> SINDSKILSLQNKKNALVDTSGYNAEVRLEGDVQVNTIYTNDFKLSSSGDKIIVNLNNNILYSAIYENSSVSFWIKISKDLTNSHNEYTIINSIKQNSGWKLCIRNGNIEWILQDINRKYKSLIFDYSESLSHTGYTNKWFFVTITNNIMGYMKLYINGELKQSERIEDLDEVKLDKTIVFGIDENIDENQMLWIRDFNIFSKELSNEDINIVYEGQILRNVIKDYWGNPLKFDTEYYMIN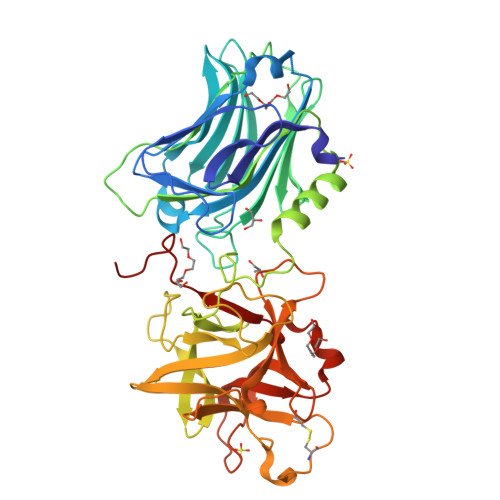YNYIDRYIAPKNNILVLVQYSDISKLYTKNPITIKSAANKNPYSRILNGDDIMFHMLYDSREYMIIRDTDTIYATQGGQCSKNCVYALKLQSNLGNYGIGIFSIKNIVSQNKYCSQIFSSFMKNTMLLADIYKPWRFSFENAYTPVAVTNYETKLLSTSSFWKFISRDPGWVEHHHHHH> GSHMEPQLVEKIIFFSDILAFSTLTEKLPVNEVVILVNRYFSICTRIISAYGGEVTKFIGDCVMASFTKEQGDAAIRTSLDIISELKQLRHHVEATNPLHLLYTGIGLSYGHVIEGNMGSSLKMDHTLLGDAVNVAARLEALTRQLPYALAFTAGVKKCCQAQWT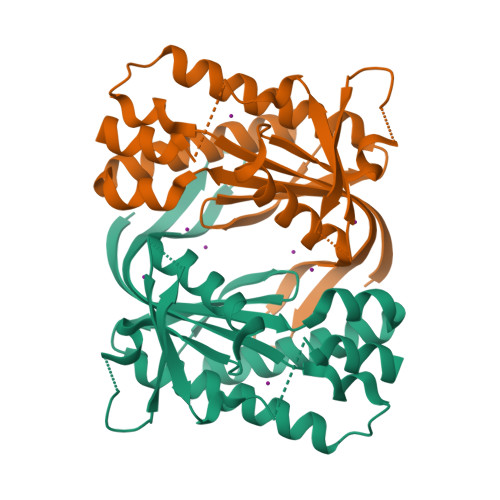FINLGAHQVKGKQEAIEVYTVNEAQKYYDTLQITQLIRQTLENDK>[6x]MSALKDKTGRFVVLDKNASNYESLVDQEMNNVYERVMKLDPNQVEFLQAFHEILYSLKPLFMEEPKYLPIIETLSEPERAIQFRVCWLDDNGVQRKNRCFRVQYNSALGPYKGGLRFHPSVNLSIVKFLGFEQIFKNSLTGLSMGGGKGGSDFDPKGKSDNEILKFCQAFM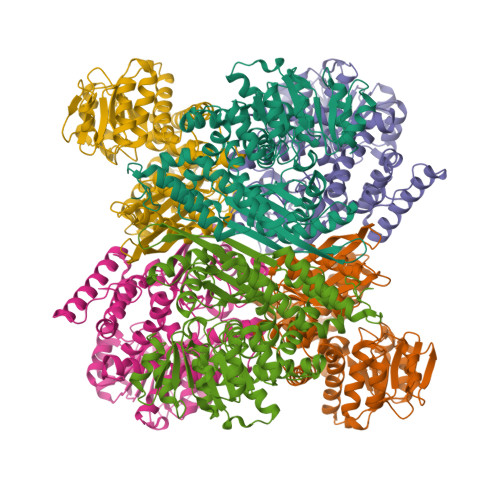NELYRHIGPCTDVPAGDIGVGGREIGYLYGQYKKIVNSFNGTLTGKNVKWGGSNLRVEATGYGLVYFVLEVLKSLNIPVEKQTAVVSGSGNVALYCVQKLLHLNVKVLTLSDSNGYVYEPNGFTHENLEFLIDLKEEKKGRIKEYLNHSSTAKYFPNEKPWGVPCTLAFPCATQNDVDLDQAKLLQKNGCILVGEGANMPSTVDAINLFKSNNIIYCPSKAANAGGVAISGLEMSQNFQFSHWTRETVDEKLKEIMRNIFIACSENALKYTKNKYDLQAGANIAGFLKVAESYIEQGCF Serpins (1–3) are folded into a metastable conformation with a surface-exposed reactive center loop. Once the reactive loop is recognized and cleaved by the target protease, a dramatic conformational change occurs, with the incorporation of the reactive loop into the middle of the central β-sheet A and a translocation and inactivation of the covalently linked protease. The Z mutation (E342K) of α1-antitrypsin (α1-AT),4 carried by 4% of Northern Europeans, predisposes to the early onset of emphysema due to decreased functional α1-AT in the lung and to liver cirrhosis due to accumulation of α1-AT polymers in the endoplasmic reticulum of hepatocytes. Glu-342 is located at the top of strand 5 of central β-sheet A (s5A) in the P17 position (active site residue termed P1) at the base of the reactive center loop and forms a highly conserved salt bridge to Lys-290 and a hydrogen bond to Thr-203.

To further understand the conformation of Z α1-AT, we carried out crystallization screens on various α1-AT mutants expressed in E. coli and on glycosylated Z α1-AT expressed in Drosophila cells. Only crystals from glycosylated recombinant Z α1-AT yielded a good diffraction data set at 3.3 Å, and the structure was solved by molecular replacement. Unexpectedly, the overall structure of Z α1-AT largely resembles that of wild type with a closed 5-stranded β-sheet A and a fully exposed reactive center loop. Although the overall resolution of the structure is modest, the electron density map around Lys-342 is unambiguous as shown in Fig. 5b. It appears that the positively charged side chain has a minimal effect on overall packing around the hinge region of Z α1-AT. Nevertheless, superposition of wild type α1-AT with that of Z α1-AT reveals subtle differences between Z and wild type α1-AT, with a change in orientation of the reactive loop and a slight shift of s5A at the top half of β-sheet A. The reactive loop of Z α1-AT is fully extended, and in the wild type α1-AT structure and most other inhibitory serpins the reactive center loop characteristically takes a U turn around P17 and P16 with residues P15 and P14 poised to enter the central β-sheet. Close inspection of crystal packing reveals that the P13 and P12 residues of the reactive loop from one Z α1-AT molecule are packed against either hH or hE from a symmetry-related molecule. It is likely that both the crystal packing and the increased flexibility around s5A allow Z α1-AT to crystallize in a native-like conformation with a relatively extended reactive loop. As Z α1-AT is largely active, it must have the ability to adopt a normal inhibitory conformation for protease inhibition as seen in its crystal structure shown here. This structure of Z α1-AT allows us to propose that Z α1-AT has a labile s5A and equilibrates between a native inhibitory conformation as shown in its crystal structure and an aberrant conformation with s5A only partially incorporated into the central β-sheet.

>[2x]RSHHHHHHGDAAQKTDTSHHDQDHPTFNKITPNLAEFAFSLYRQLAHQSNSTNIFFSPVSIATAFAMLSLGTKADTHDEILEGLNFNLTEIPEAQIHEGFQELLRTLNQPDSQLQLTTGNGLFLSEGLKLVDKFLEDVKKLYHSEAFTVNFGDTEEAKKQINDYVEKGTQGKIVDLVKELDRDTVFALVNYIFFKGKWERPFEVKDTEEEDFHVDQVTTVKVPMMKRLGMFNIQHCKKLSSWVLLMKYLGNATAIFFLPDEGKLQHLENELTHDIITKFLENEDRRSASLHLPKLSITGTYDLKSVLGQLGITKVFSNGADLSGVTEEAPLKLSKAVHKAVLTIDKKGCEAAGAMFLEAIPRSIPPEVKFNKPFVFLMIEQNTKSPLFMGKVVNPTQK N-(ethoxycarbonyl)-L-leucyl-N-[(1R,2S,3S)-1-(cyclohexylmethyl)-2,3-dihydroxy-5-methylhexyl]-L-leucinamide | C29 H55 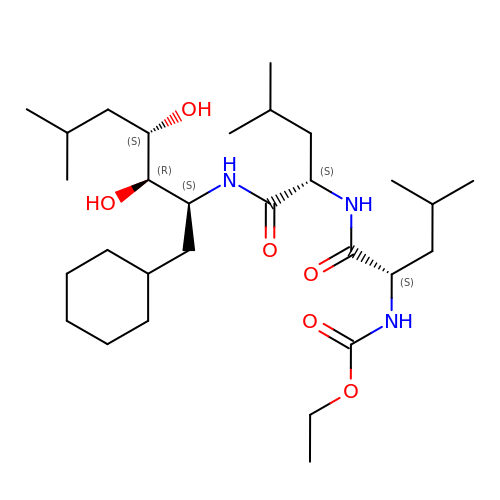N3 O6 | OAFXIYWBKGSXMT-WBAQKLHDSA-N>GSSHHHHHHSQDPAPTLLTTQFSNPAEVTDFVVYKGNGVKGLSETGIKALPEQYIQPLEERLINKFVNETDEAIPVIDMSNPDEDRVAEAVCDAAEKWGFFQVINHGVPLEVLDDVKAATHKFFNLPVEEKRKFTKENSLSTTVRFGTSFSPLAEQALEWKDYLSLFFVSEAEAEQFWPDICRNETLEYINKSKKMVRRLLEYLGKNLNVKELDETKESLFMGSIRVNLNYYPICPNPDLTVGVGRHSDVSSLTILLQDQIGGLHVRSLASGNWVHVPPVAGSFVINIGDAMQIMSNGLYKSVEHRVLANGYNNRISVPIFVNPKPESVIGPLPEVIANGEEPIYRDVLYSDYVKYFFRKAHDGKKTVDYAKI[2x]

Recently, the actual enzyme involved was identified and characterized from A. thaliana and was designated as feruloyl-CoA 6’-hydroxylase (F6’H1)10. The product 6’-hydroxyferuloyl-CoA is converted into a simple coumarin scopoletin via spontaneous trans/cis isomerization and lactonization. The activity of F6’H1 is entirely dependent on the presence of 2-oxoglutarate and the Fe (II) ion. Sequence alignment showed that F6’H1 contains the conserved Fe(II)-binding motif (His-X-Asp-Xn-His) and the 2-oxoglutarate C5 carboxy group binding motif (Arg-X-Ser).

In this study, we determined the crystal structure of F6’H1 apo enzyme by molecular replacement and also generated a homology model of C2’H structure. Diffraction analysis of the colorless plate shaped F6’H1 crystals indicated that they belonged to space group C2, with unit-cell parameters a = 193.22 Å b = 54.55 Å, c = 78.82 Å and γ = 111.5°. The F6’H1 structure consists of residues A15-A343, B15-B141, B144- B344, 28 solvent molecules modeled as water and two sodium ions. As expected the F6’H1 structure closely resembles the structure of the A. thaliana Anthocyanidin synthase (ANS) search model. Like other members of this class of enzymes the structure contains an N-terminal DIOX_N (PF14226) domain, residues 62-172 linked to a C-terminal 2OG-FeII_OXY (PF03171) domain, residues 212 – 312 that contains the catalytic site22. Strands β1, β2, β10, β7, β12, β5, β4 and β3 form an 8-stranded mixed β sheet, which assumes a β jellyroll fold common to this family of enzymes. Sheets S1 and S2 together form a large (2,309 Å3) hydrophobic pocket that contains the catalytic site23. The F6’H1 substrate binding pocket is contained within the C-terminal 2OG-FeII_OXY domain with its dominate feature being the 2-HIS-1-carboxylate facial triad (residues HIS 235, ASP 237 and HIS 293) that is involved in iron binding. However, in the apo structure reported here the iron site is occupied by a sodium ion. Many of the key residues (ASN 218, TYR 220, ARG 303 and SER 305) involved in binding the 2OG co-substrate are structurally conserved in the F6’H1 structure.> MNTPEHMTAVVQRYVAALNAGDLDGIVALFADDATVEGGVGSEPRSGTAAIREFYANSLKLPLAVELTQEVRAVANEAAFAFTVSFEYQGRKTVVAPINHFRFNGAG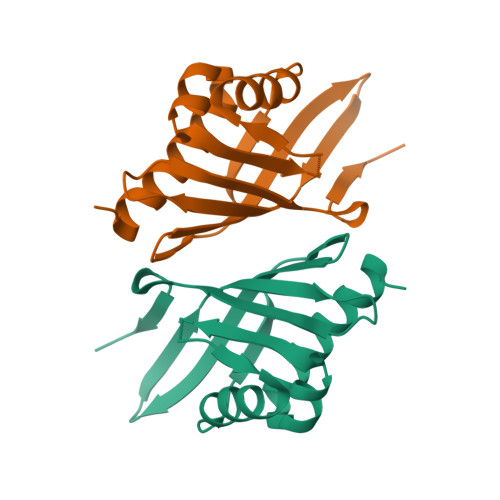KVVSMRALFGEKNIHAGA>SHMKSFFDKKRSERISNGGFRPAAPNLAGAVEFSDVKTLLKEWITTISDPMEEDILQVVRYCTDLIEEKDLEKLDLVIKYMKRLMQQSVESVWNMAFDFILD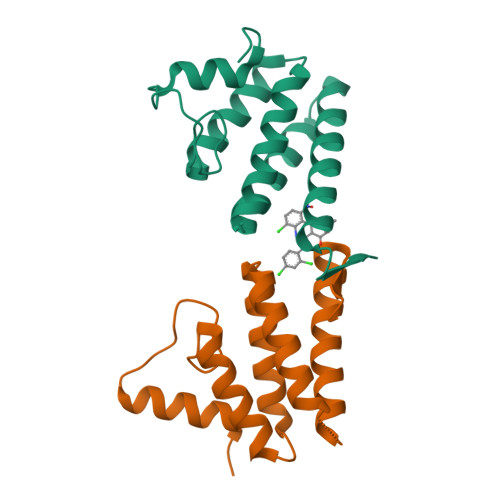NVQVVLQQTYGSTLKVT[2x]> GKGG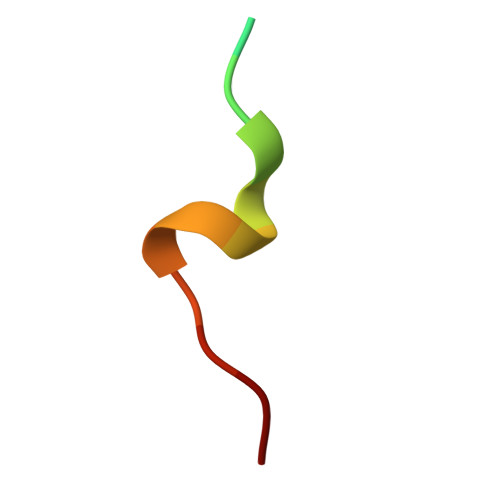QGSIMSWFAKK>MGAVFKLMKSDFYEREDFMGEVEDMITLKDIFGTETLKRSILFSFQYELDFLLRQFHQNVENITIVGQKGTIMPIEARAMDATLAVILKKVKLIEITMPPFASHHTKLIINFYDNGECKIFLPSNNFTSMETNLPQQVCWCSPLLKIGKEGLPVPFKRSLIEYLNSYHLKDIDELITKSVEEVNFAPLSELEFVYSTPSKFQSSGLLSFYNKLEKLSAGTSASDTAKHYLCQTSSIGTSLSRARDENLWTHLMIPLFTGIMSPPAKDTAGRKKAEILPTNSLINEYSQRKIKPYIIFPTEQEFVTSPLKWSSSGWFHFQYLQKKSYYEMLRNKFKVFYKQDPAMVTRRRGTTPANSKFYMHCATNS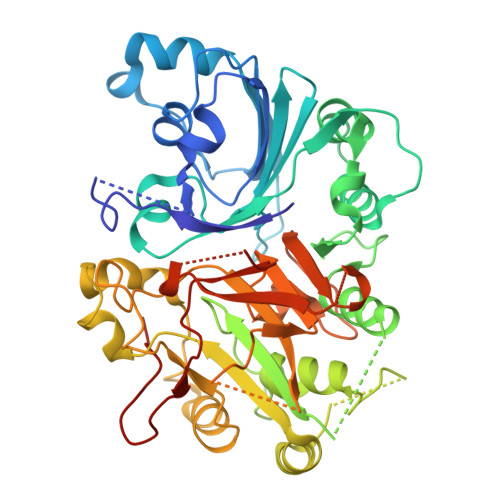AGPCDASQVFKELEWCLYTSANLSQTAWGTVSRKPRNYEAGVLYHSRRLANTRKVTCRTFTRDRRGCAGNPTHVAVPFTLPVIPYDLAEDECFCLALHHHHHHH[4x]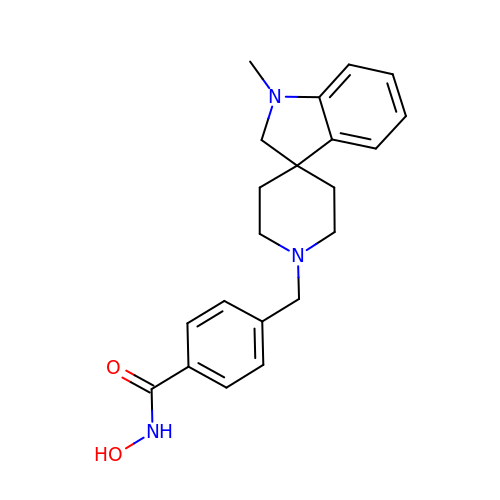N-hydroxy-4-[(1-methyl-1,2-dihydro-1'H-spiro[indole-3,4'-piperidin]-1'-yl)methyl]benzamide | C21 H25 N3 O2 | KRAFQDJIYXJLQM-UHFFFAOYSA-N> MAHHHHHHVDDDDRMGKPQKADSNNSSKSLQSAGFTAGLTYSQLMTLKDAMLQLDPNAKTWMDIAGRPEDPVEIALYQPSSGCYIHFFREPTDLKQFKQDAKYSHGID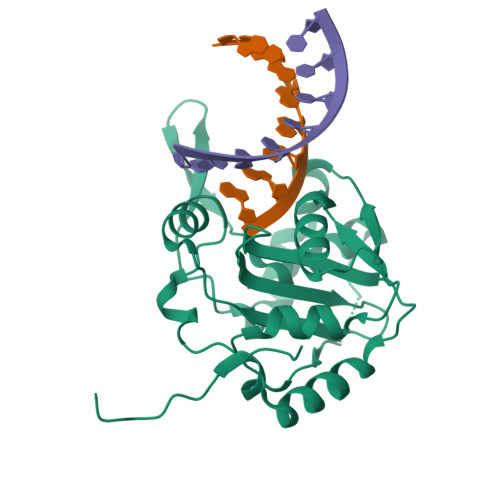VTDLFATQPGLTSAVIDALPRNMVITCQGSDDIRKLLESQGRKDIKLIDIALSKTDSRKYENAVWDQYKDLCHMHTGVVVEKKKRGGKEEITPHCALMDCIMFDAAVSGGLNTSVLRAVLPRDMVFRTSTPRVVL> HGYIESPPSRQQHCGAEQKPDNPSSAKCDEAFANYRAAGGQNSHWYNFMSVVAHHEGRKVVKGTEHVCGFDGETWNPAPYDTPANWPVTSFNSGQQTFVWDISYGPHFSDTEELVFYITKPGFSFDPTRELTWADFEDQPFCDESIVPGDFSTNSAVEADMANSHINVTCNVPSRSGRHVIFAEWG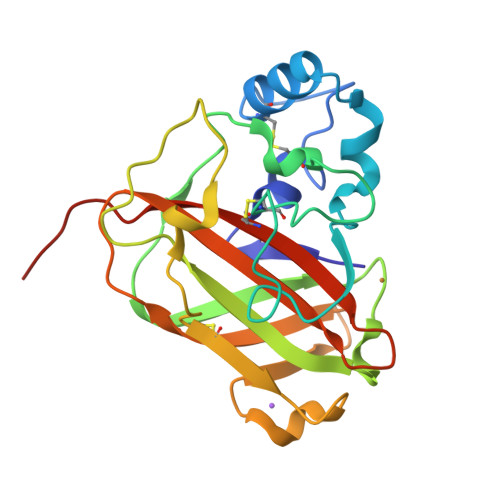RNEHTYERFFSCVDVDFGWSHPNFEK>[2x]MSSSSPGEPLEPTDQDLDVLLKNLGNLVTPMALRVAATLRLVDHLLAGADTLAGLADRTDTHPQALSRLVRHLTVVGVLEGGEKQGRPLRPTRLGMLLADGH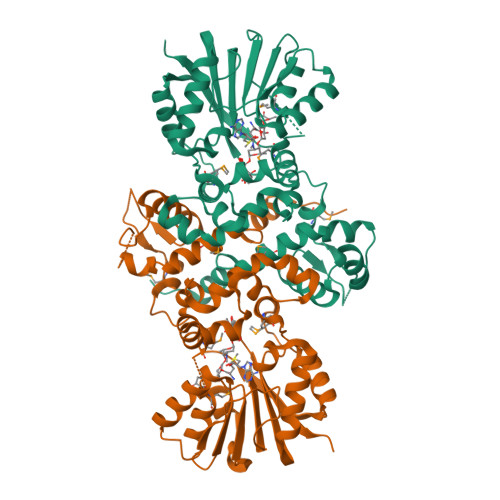PAQQRAWLDLNGAVSHADLAFTGLLDVVRTGRPAYAGRYGRPFWEDLSADVALADSFDALMSCDEDLAYEAPADAYDWSAVRHVLDVGGGNGGMLAAIALRAPHLRGTLVELAGPAERARRRFADAGLADRVTVAEGDFFKPLPVTADVVLLSFVLLNWSDEDALTILRGCVRALEPGGRLLVLDRADVEGDGADRFFSTLLDLRMLTFMGGRVRTRDEVVDLAGSAGLALASERTSGSTTLPFDFSILEFTAVSEEAAPAAQASEALPAQE>SIDVESVNQKLDDVIAALARIEAD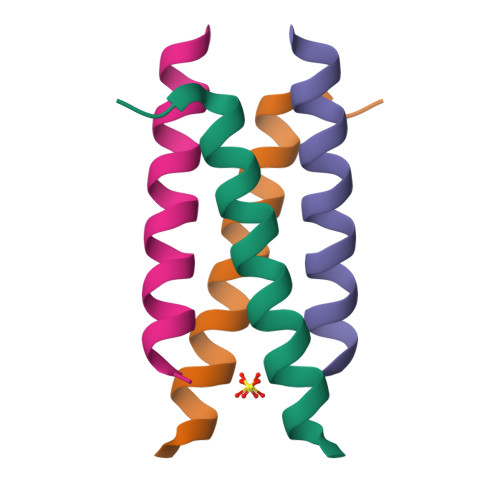RKNSNEQMV[2x]>[8x]GG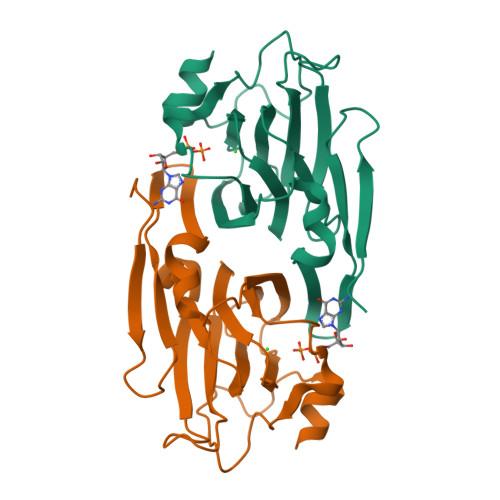HMEIKFNIEESKILNGVYIITPNKFSDLRGDIWTAFTDEYLSNLVPNGIKFKHDKFINSHFNVLRGIHGDVKTYKLVTCVYGEVHQVVVDCRKDSPTYLKWEKFIISPRNQQLILLPPNMGNSHYVSSKEAVYYYKLAYEGEYLDAPDQFTYAWNDERIAIDWPTNSPILSERDILAMNKDK>MSFTPANRAYPYTRLRRNRRDDFSRRLVRENVLTVDDLILPVFVLDGVNQRESIPSMPGVERLSIDQLLIEAEEWVALGIPALALFPVTPVEKKSLDAAEAYNPEGIAQRATRALRERFPELGIITDVCLCEFTTHGQCGILDDDGYVLNDVSIDVLVRQALSHAEAGAQVVAPSDMMDGRIGAIREALESAGHTNVRVMAYSAKYASAYYGPFRDAVGSASNLGKGNKATYQMDPANSDEALHEVAADLAEGADMV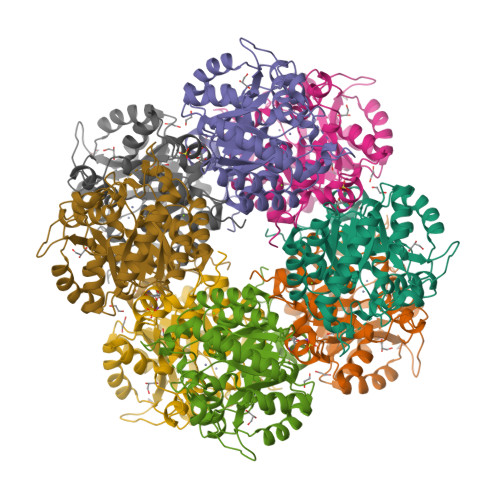MVKPGMPYLDIVRRVKDEFRAPTFVYQVSGEYAMHMGAIQNGWLAESVILESLTAFKRAGADGILTYFAKQAAEQLRRGR[2x]5-(4-FLUOROPHENYL)-3,3-DIMETHYL-INDOLIN-2-ONE 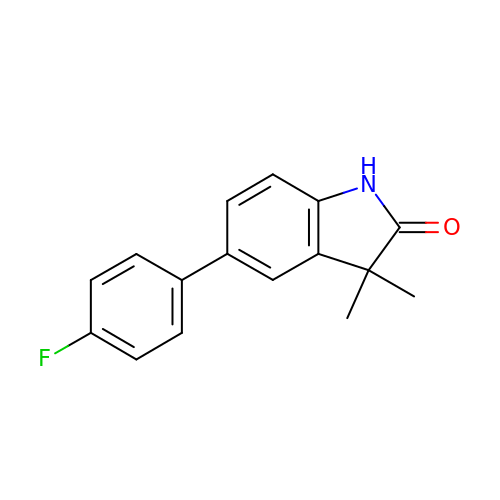| C16 H14 F N O | VXOIAVBQYFDIBS-UHFFFAOYSA-N>MGSSHHHHHHSSGLVPRGSHMTGAGLRWKHTSSLKVANEPVLAFTQGSPERDALQKALKDLKGRMEAIPCVVGDEEVWTSDVQYQVSPFNHGHKVAKFCYADKSLLNKAIEAALAARKEWDLKPIADRAQIFLKAADMLSGPRRAEILAKTMVGQGKTVIQAEIDAAAELIDFFRFNAKYAVELEGQQPISVPPSTNSTVYRGLEGFVAAISPFNFTAIGGNLAGAPALMGNVVLWKPSDTAMLASYAVYRILREAGLPPNIIQFVPADGPLFGDTVTSSEHLCGINFTGSVPTFKHLWKQVAQNLDRFHTFPRLAGECGGKNFHFVHRSADVESVVSGTLRSAFEYGGQKCSACSRLYVPHSLWPQIKGRLLEEHSRIKVGDPAEDFGTFFSAVIDAKSFARIKKWLEHARSSPSLTILAGGKCDDSVGYFVEPCIVESKDPQEPIMKEEIFGPVLSVYVYPDDKYKETLQLVDSTTSYGLTGAVFSQDKDVVQEATKVLRNAAGNFYINDKSTGSIVGQQPFGGARASGTNDKPGGPHYILRWTSPQVIKETHKPLGDWSYAYMQ[2x]

The aromatic ring system of these compounds is able to include lysine and arginine side chains, supported by one or two phosphate groups that are attached to the half-moon-shaped molecule. Furthermore, we solved crystal structures of two different tweezer variants in complex with the enzyme Δ1-Pyrroline-5-carboxyl-dehydrogenase (P5CDH) and found that the tweezers are bound to a lysine and methionine side chain, respectively. Therefore, P5CDH was chosen as a target for the systematic analysis of co-crystallization with two different tweezer molecules, the diphosphate tweezer CLR01, which was also used for the 14-3-3 structures, and a monophosphate tweezer, where one phosphate group is replaced by a sterically less-demanding hydroxyl group. In both crystals, only one tweezer molecule is seen in the asymmetric unit despite the presence of two and four monomers of P5CDH, respectively, revealing an asymmetric binding mode of the tweezer to P5CDH, depending on the non-equivalent environment of the tweezer binding sites in the monomers.

Co-crystallizing P5CDH with the monophosphate tweezer (MPT) instead of the diphosphate tweezer CLR01 resulted in a different crystal form that diffracted to 1.2 Å, with the physiological dimer (instead of a tetramer) in the asymmetric unit. Very clear electron density for a single MPT molecule was found next to Lys402 of monomer A, with the single phosphate group at the ε-amine of the side chain of Lys402 pointing into solvent and the hydroxyl group facing the α-helix. In addition, H-bonds between the phosphate group of the tweezer to the side chain of Lys52 of the neighbor protein molecule facilitate the formation of a noncovalent supramolecular bridge between the protein containing the hosted lysine side chain and the neighbor molecule. A superimposition of monomer A to monomer B shows the putative clash of the MPT molecule with Pro120 of the symmetry-related molecule and the lack of positive charge to stabilize the tweezer at this position. Since at least one MPT was bound at Lys402 of P5CDH, and since the solvent channels seem to be sufficiently large, this raises the question of why CLR01 did not bind at this position. A superimposition of CLR01 on the P5CDH-MPT crystal structure shows that the second phosphate group would clash with the protein surface, illustrating the more demanding sterical requirements for CLR01 binding. In contrast, the MPT in the P5CDH complex structure is actually found at a lysine side chain within an alpha-helix, where the smaller hydroxyl group that replaces one of the phosphates can readily be accommodated. The surface around P5CDH-Lys402 bound by the monophosphate tweezer is also strongly positively charged by the ε-amine of the clamped lysine and the neighboring arginines (Arg399 and the symmetry-related Lys5), and shows a surrounding “moat” that accommodates the ring system.>[6x]MSQEIRQNEKISYRIEGPFFIIHLMNPDNLNALEGEDYIYLGELLELADRNRDVYFTIIQSSGRFFSSGADFKGIAKAQGDDTNKYPSETSKWVSNFVARNVYVTDAFIKHSKVLICCLNGPAIGLSAALVALCDIVYSINDKVYLLYPFANLGLITEGGTTVSLPLKFGTNTTYECLMFNKPFKYDIMCENGFISKNFNMPSSNAEAFNAKVLEELREKVKGLYLPSCLGMKKLLKSNHIDAFNKANSVEVNESLKYWVDGEPLKRFRQLGSKQRKHRL

A prominent example is peroxisomal matrix proteins, most of which depend on the targeting factor Pex5 to localize and function correctly. One such example is the yeast Eci1 (Δ3, Δ2-enoyl-CoA isomerase 1), an enzyme that is essential for the β-oxidation of unsaturated fatty acids in peroxisomes. Although Eci1 contains a PTS1, its targeting to peroxisomes can occur independently of this signal. Using cryo-electron microscopy (cryo-EM), we resolved the structure of the Pex5–Eci1 complex, revealing a novel binding interface in addition to the PTS1-binding interface.

The cryo-EM reconstruction of the Pex5–Eci1 complex dataset revealed that Eci1 forms a hexamer, with a single subunit bound to a Pex5 monomer. Although the Eci1 hexamer was readily resolved to high resolution, the electron density of the bound Pex5 was poorly resolved and showed conformational heterogeneity relative to Eci1. The maps from this subset were refined to 2.7 Å (1 Å=0.1 nm) globally, whereas Pex5 and the interface were resolved to 2.9 Å after local refinement of this region. At the atomic level, Eci1 consists of an N-terminal core domain (M1–N200) with a spiral fold topology and a C-terminal region (M201–L280) forming an α-helical trimerization domain. In the trimerization domain, three Eci1 subunits formed a characteristic trimeric disk with strong interactions between the three subunits. Two of these trimeric disks combined to create a hexamer. Given that the 3D refinement was performed without applying symmetry, the six Eci1 subunits exhibited variations in the resolved residues. Specifically, five subunits contained residues I5–Q270, E4–Q270, I5–Q270, E4–Q270 and I5–Q270. The Pex5-bound Eci1 subunit contains a distinct segment at its C-terminal end (268FRQLGSKQRKHRL280), highlighted with a black circle and labeled as PTS1 in Fig. 4A. Electron density for this C-terminal segment, including the PTS1, was absent in the other five Eci1 subunits that did not bind Pex5.6-(2-{3-[3-(dimethylamino)prop-1-yn-1-yl]-5-fluorophenyl}ethyl)-4-methylpyridin-2-amine 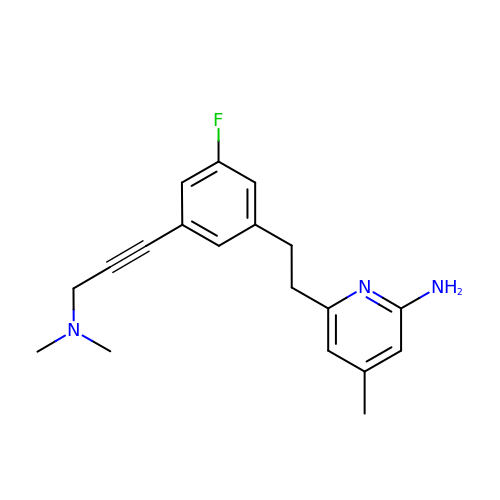| C19 H22 F N3 | YSCHBYRLJPUGBG-UHFFFAOYSA-N> KVTMNDFDYLKLLGKGTFGKVILVREKATGRYYAMKILRKEVIIAKDEVAHTVTESRVLQNTRHPFLTALKYAFQTHDRLCFVMEYANGGELFFHLSRERVFTEERARFYGAEIVSALEYLHSRDVVYRDIKLENLMLDKDGHIKITDFGLCKEGISDGATMKTFCGTPEYLAPEVLEDNDYGRAVDWWGLGVVMYEMMCGRLPFYNQDHERLFELILMEEIRFPRTLSPEAKSLLAGLLKKDPKQRLGGGPSDAKEVMEHRFFLSINWQDVVQKKLLPPFKPQVTS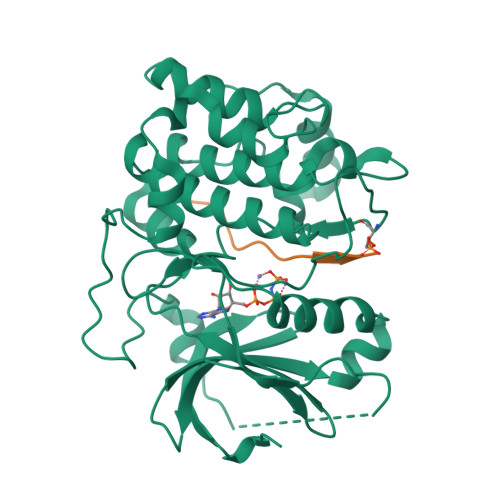EVDTRYFDDEFTAQSITITPPDRYDSLGLLELDQREEQEMFEDFDYIADW;> GRPRTTSFAE>[2x]MANVLMIGFPGEGHINPSIGVMKELKSRGENITYYAVKEYKEKITALDIEFREYHDFRGDYFGKNATGDEERDFTEMLCAFLKACKDIATHIYEEVKHESYDYVIYDHHLLAGKVIANMLKLPRFSLCTTFAMNEEFAKEMMGAYMKGSLEDSPHYEEYQQLAETLNADFQAEIKKPFDVFLADGDLTIVFTSRGFQPL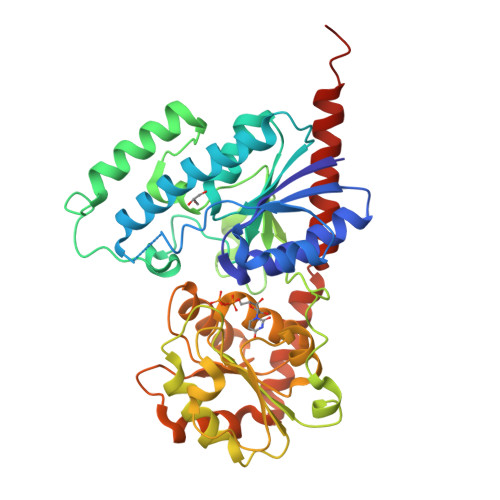AEQFGERYVFVGPSITERHGNNDFPFDQIDNENVLFISMGTTFNNQKQFFNQCLEVCKDFDGKVVLSIGKHIKTSELNDIPENFIVRPYVPQLEILKRASLFVTHGGMNSTSEGLYFETPLVVIPMGNDQFVVADQVEKVGAGKVIKKEELSESLLKETIQEVMNNRSYKEKAKEIGQSLKAAGGSKKAADSILEAVKQKTQSANAALEHHHHHH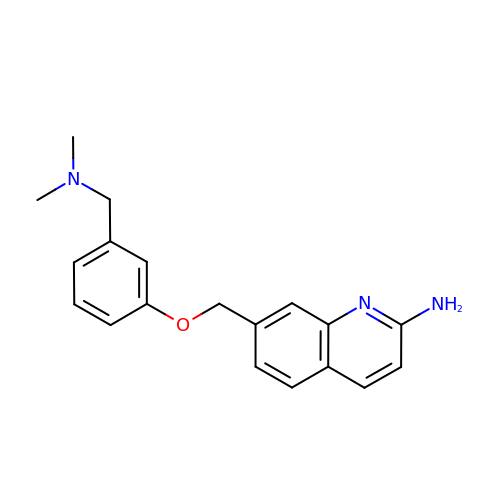7-[[3-[(dimethylamino)methyl]phenoxy]methyl]quinolin-2-amine | C19 H21 N3 O | NTASSNARMLLQTN-UHFFFAOYSA-N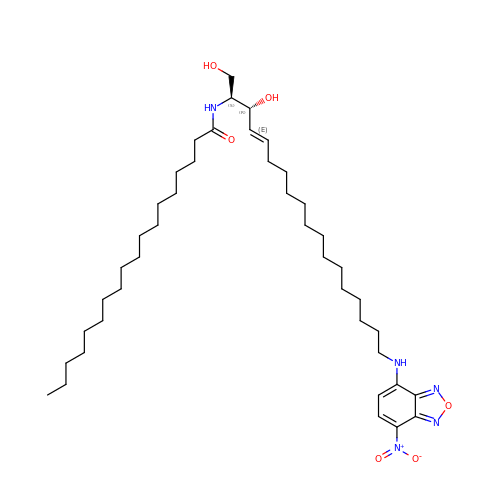~{N}-[(~{E},2~{S},3~{R})-18-[(4-nitro-2,1,3-benzoxadiazol-7-yl)amino]-1,3-bis(oxidanyl)octadec-4-en-2-yl]octadecanamide | C42 H73 N5 O6 | VBDLKCVULNLCGA-HVRWNUQKSA-N> MAATPGTRTTPADEAREAAVEKALAALDLDAKARLLSGQDMWTLPALPEIGLASLVMSDGPIGVRGVRWTADDPSVALPSPTALAATWDPGLARRAGVLLAQEARRKGVHVLLAPTVNLHRSPLGGRHFEAYSEDPYLTGEIGSGYVTGVQAGGVGTTVKHFVANDAETDRFTVNNLVSARALRELYLAPFEAIVANAHPWGIMTAYNQVNGSTMTEHRYLVNEVLRGEWGFDGFNVSDWLAARSTTGALTGGLDVAMPGPATVYGEPLAAAVRAGEVTESLLDEAVRRVLRLAARVGILEGAAPAVTELPAPVDGEALAREIARRSFVLVRNEVRDGRAALPLEQGATVALIGAAARDARVLGGGSATVFPARVVSPLDGLTAALPEGAPTYALGADPNEELAVADTGFTLRAVCRDASGTVIGTRSAPNGHI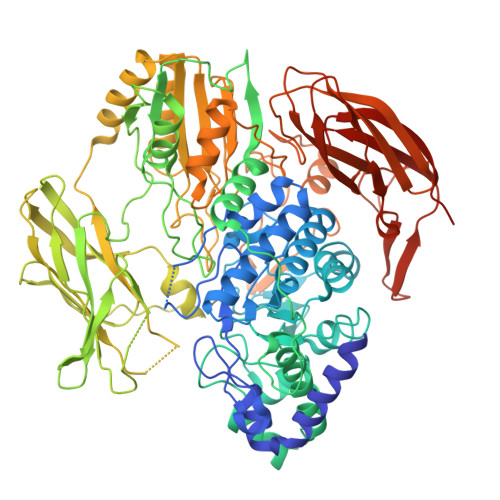QWMGSDLPDGVTHATLHSVELTGTFTPRETGTHTFGVKGLGAYTLTVDGTTHFDGVRTTDTDDPFVSFFGAPVPLAEVELTEGTPLEVSLTHVVELAADAPITMLAFSLCHQEPQRDPDELIAEAVEAARAADTAVVVVATTERVESEGFDRKDLRLPGRQDDLVRAVAAANPATVVVVNAGSPVELPWREDVAAVLLTWFPGQEGGAALAEVLTGAHEPGGRLPTTWGSLTGAPVTQVTPTAGELVYDEGVFIGYRAWDKEDRTPTYPFGHGLGYTDWTYESLDVTGTTATVRVRNTGTREGRETVQLYLAPTTADENRPTRWLAGFATVEAAPGETAEAVVRLPRRAFEIWDETTGAWVYVTGSYEVAAGRSIADRRTRVTIEAPKLAAALEHHHHHH(4S)-4-[(1R)-1,2-dihydroxyethyl]-N,N-dimethyl-2-oxo-11,16-dioxa-3-azatricyclo[15.3.1.1~6,10~]docosa-1(21),6(22),7,9,17,19-hexaene-19-carboxamide 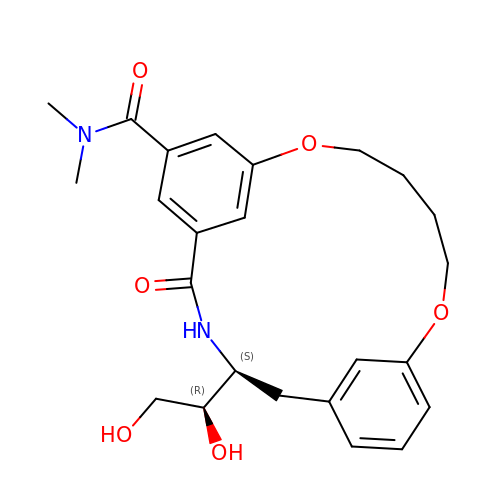| C24 H30 N2 O6 | YKCXDIPNOWOCAE-VXKWHMMOSA-N> AMYHFQNKFVSKANGQSATAKSAFNSASRIKDFKENEFKDYSNKQCDYSEILLP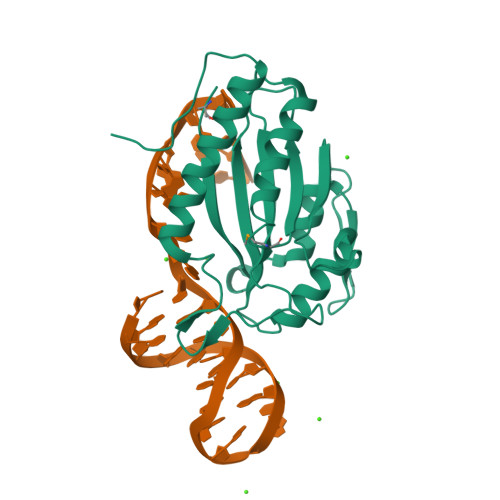NNADDKFKDREYLWNKVHDVENRKNSQVAREIIIGLPNEFDPNSNIELAKEFAESLSNEGMIVDLNIHKINEENPHAHLLCTLRGLDKNNEFEPKRKGNDYIRDWNTKEKHNEWRKRWENVQNKHLEKNGFSVRVSADSYL>[48x]MAAVINTNYLSLVAQNNLNKSQSSLGTAIERLSSGLRINSAKDDAAGMAIANRFTANVRGLTQAARNANDGISLAQTTEGAASEVNTHLQRIRELTVQASNGSYSQEQLDSVQGEINQRLADIDRISEQTDFNGVKVLSDSAKPLTLQVGANDGETITLNLSEISVKTLGLDGFNVNGKGVTQNRSATVTDVIAQGGTLQGDGTYKATTTFNAASAETVLSKLEDGNTVAVGGGATYTYDAAKGNFTYTKTVDTTVGADVTALANKIKPSSGTISGSYEISTGKSASFDVDAAGKITIGGNAAFLNADGELTTNDASGALTQATLDDVLTSVGTEANSSVTIGGTKYSHSAADELSYTAVATTADVLSAMGSSTAVSTVTLGSGITSAAVTFAIATTDSNNTWVDNKGELTDIQTFDTSYKINADTGEVTVVGDNSATAGQYASADGAKVLVGSDGKLTTETTSAGDKTTDPLKTLDAAFTKLDKLTGELGAVQNRLESTIANLNNVVNNLSSARSRIQDADYATEVSNMSKAQILQQAGTSVLAQANQVPQTVLSLLR

The rotating flagellar filament primarily functions as a propeller, acting as an Archimedean screw, and supercoiling of the filament is essential as rotations of a straight filament do not generate thrust. Here, we show the atomic cryo-electron microscopy structures for flagellar filaments from enterohemorrhagic Escherichia coli O157:H7, enteropathogenic E. coli O127:H6, Achromobacter, and Sinorhizobium meliloti, where the outer domains dimerize or tetramerize to form either a sheath or a screw-like surface. A shared feature in all four structures is the formation of symmetrical homodimers between the outer domains of flagellin subunits, with one outer domain rotated 180° relative to the other. These symmetrical dimers are the result of outer domains being able to adopt either an “up” or “down” conformation.

We discovered the existence of non-canonical flagellar filaments in Achromobacter sp. MFA1 R437,38, a soil bacterium that was identified as a cell culture contaminant. Like the EHEC H7, the Achromobacter ODS is also formed by interactions between flagellins that are five, 11, and 27 subunits away. However, there are four flagellins in the Achromobacter ASU, with two up and two down conformations. The key distinction is that all of the EHEC H7 Sn:Sn+27 dimers form at a single radius while the Achromobacter Sn:Sn+27 dimers occur at two different radii. Consequently, the Achromobacter outer domain exists in four conformations and the filament has four flagellins in the ASU with an axial rise and twist for the outer domains that is four times larger than that of the flagellar core. This tetrameric symmetry is characterized by two 4-start helices that occur at different radii. The ODS surrounding the EHEC H7 and Achromobacter flagellar filaments produces an intermediate waveform that is not adopted by the “canonical” S. typhimurium and E. coli K-12 H48 flagellar filaments. A notable difference was the greater stability of the intermediate waveform in Achromobacter and wild-type EHEC H7 filaments compared to the FF mutant filaments, which underwent frequent polymorphisms.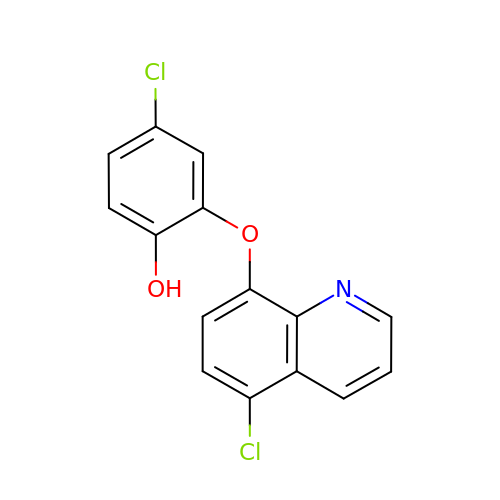4-chloro-2-[(5-chloroquinolin-8-yl)oxy]phenol | C15 H9 Cl2 N O2 | PXDPCRTVJVDTRN-UHFFFAOYSA-N>[3x]GAMGNKEKADQQKAITDIVALENALDMYKLDNSVYPTTDQ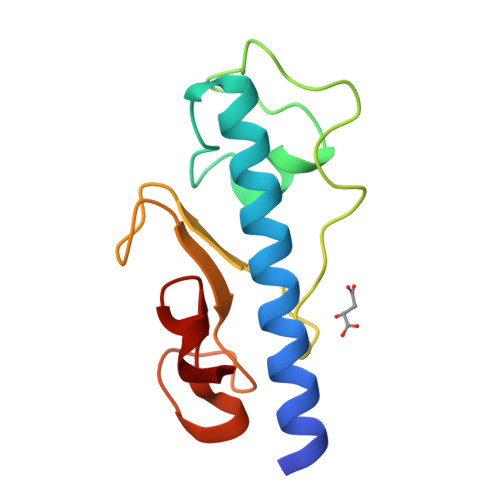GLEALVTKPSSPEPRNYRNGGYIKRLPKDPWGNEYQYMSPGDKGTIDIFTLGADGQEGGEGAAADIGNWNMQDFQ> PADLSGTWTLLSSDNFEGYMLALGIDFATRKIAKLLKPQKV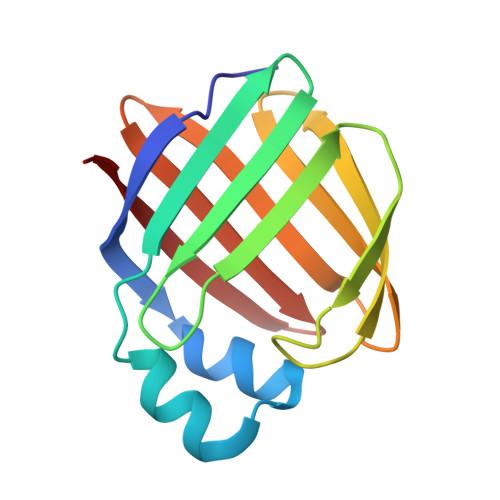IEQNGDSFTIHTNSSLRNYFVKFKVGEEFDEDNRGLDNRKCKSLVIWDNDRLTCIQKGEKKNRGWTHWIEGDKLHLEMFCEGQVCKQTFQRA> GSRRASVGSHRFKVYNYKSPTFCEHCGTLLWGLARQGLKCDACGMNVHHRCQTKVANLCEFIV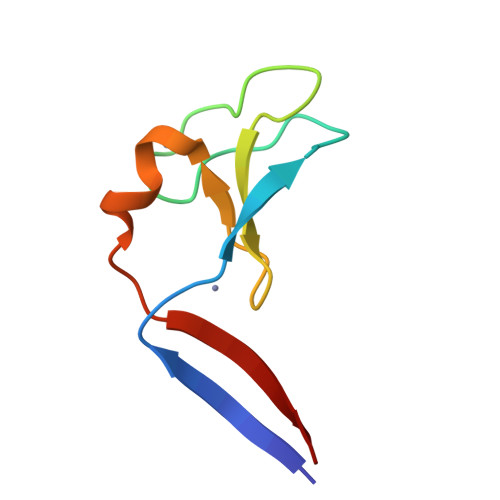TD> MHHHHHHAVRASEISRVYEAYPEKKATLYFLVLGFLALIVGSLFGPFQALNYGNVDAYPLLKRLLPFVQSYYQGLTLHGVLNAIVFTQLFAQAIMVYLPARELNMRPNMGLMWLSWWMAFIGLVVAALPLLANEATVL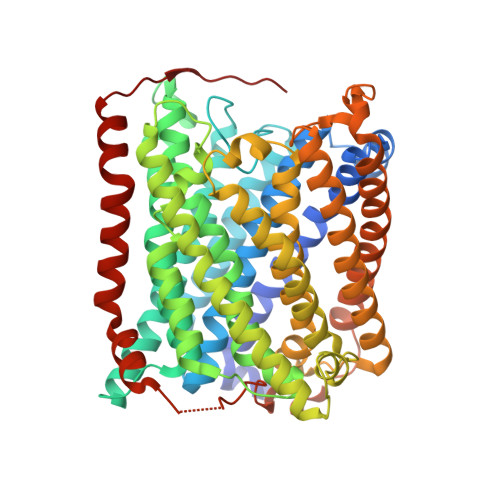WTFYPPLKGHWAFYLGASVFVLSTWVSIYIVLDLWRRWKAANPGKVTPLVTYMAVVFWLMWFLASLGLVLEAVLFLLPWSFGLVEGVDPLVARTLFWWTGHPIVYFWLLPAYAIIYTILPKQAGGKLVSDPMARLAFLLFLLLSTPVGFHHQFADPGIDPTWKMIHSVLTLFVAVPSLMTAFTVAASLEFAGRLRGGRGLFGWIRALPWDNPAFVAPVLGLLGFIPGGAGGIVNASFTLDYVVHNTAWVPGHFHLQVASLVTLTAMGSLYWLLPNLTGKPISDAQRRLGLAVVWLWFLGMMIMAVGLHWAGLLNVPRRAYIAQVPDAYPHAAVPMVFNVLAGIVLLVALLLFIYGLFSVLLSRERKPELAEAPLPFAEVISGPEDRRLVLAMDRIGFWFAVAAILVVLAYGPTLVQLFGHLNPVPGWRLW> PEFMVTTEPALADLQEQLYNGNEKSQLAAMSTLSTAGTEGYHLLQEFLK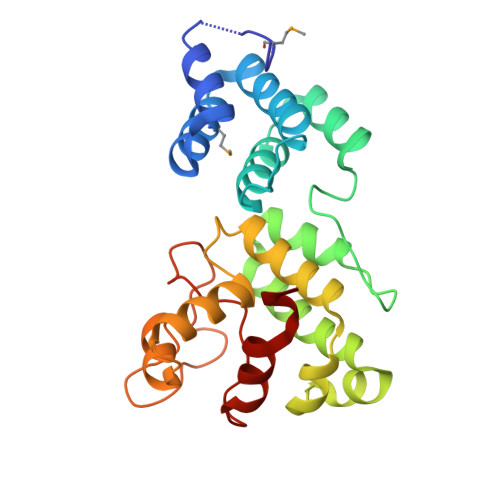DSATFSPPPAPWIRGQAYRLLFHSPEASVQAFLQQHYPQGVIPLRSDRGVDYQELAKLLVAEKFEAADRLTTQKLCELAGPLAQKRRWLYFTEVEQLPIPDLQTIDQLWLAFSLGRFGYSVQRQLWLGCGQNWDRLWEKIGWRQGKRWPRYPNEFIWDLSAPRGHLPLTNQLRGVQVLNALLNHPAWTA> MREYKLVVLGSGGVGKSALTVQFVQGIFVEKYDPTIEDSYRKQVEVDCQQCMLEILD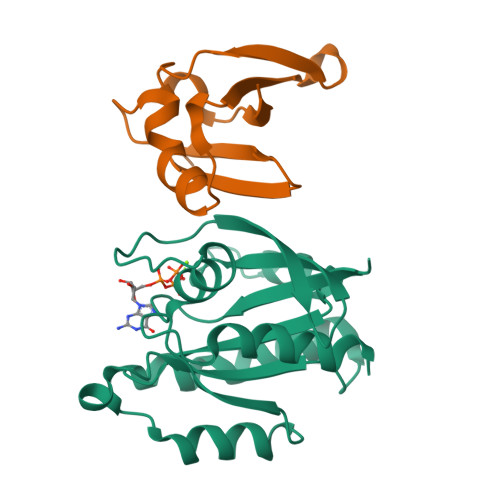TAGTEQFTAMRDLYMKNGQGFALVYSITAQSTFNDLQDLREQILRVKDTEDVPMILVGNKCDLEDERVVGKEQGQNLARQWCNCAFLESSAKSKINVNEIFYDLVRQINR;> SNTIRVFLPNKQRTVVNVRNGMSLHDCLMKALKVRGLQPECCAVFRLLHEHKGKKARLDWNTDAASLIGEELQVDFL>LYWDDLKRKLSEKLDSTDFTSTIKLLNENSYVPREAGSQKDENLALYVENEFREFKLSKVWRDQHFVKIQVKDSAQNSVIIVDKNGRLVYLVENPGGYVAYSKAATVTGKLVHANFGTKKDFEDLYTPVNGSIVIVRAGKITFAEKVANAESLNAIGVLIYMDQTKFPIVNAELSFFGHAHLGTGDPYTPGFPSFNHTQFPPSRSSGLPNIPVQTISRAAAEKLFGNMEGDCPSDWKTDSTCRMVTSESKNVKLTVSNVLKEIKILNIFGVIKGFVEPDHYVVVGAQRDAWGPGAAKSGVGTALLLKLAQMFSDMVLKDGFQPSRSIIFASWSAGDFGSVGATEWLEGYLSSLHLKAFTYINLDKAVLGTSNFKVSASPLLYTLIEKTMQNVKHPVTGQFLYQDSNWASKVEKLTLDNAAFPFLAYSGIPAVSFCFCEDTDYPYLGTTMDTYKELIERIPELNKVARAAAEVAGQFVIKLTHDVE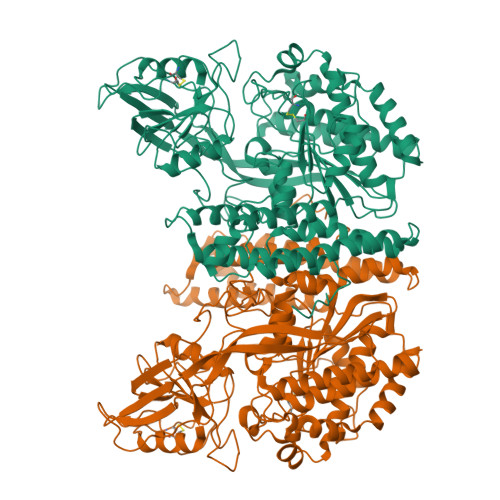LNLDYEEYNSQLLSFVRDLNQYRADIKEMGLSLQWLYSARGDFFRATSRLTTDFGNAEKTDRFVMKKLNDRVMRVEYHFLSPYVSPKESPFRHVFWGSGSHTLPALLENLKLRKQNNGAFNETLFRNQLALATWTIQGAANALSGDVWDIDNEF[2x]>[2x]GSNRRLQQTQAQVDEVVDIMRVNVDKVLERDQKLSELDDRADALQAGASQFETSAAKLKRKYW;>[2x]ALSEIETRHSEIIKLENSIRELHDMFMDMAMLVESQGEMIDRIEYNVEHAVDYVERAVSDTKKAVK;>[2x]NELEEMQRRADQLADESLESTRRMLQLVEESKDAGIRTLVMLDEQGEQLDRVEEGMNHINQDMKEAEKNLKDLGK;>ARENEMDENLEQVSGIIGNLRHMALDMGNEIDTQNRQIDRIMEKADSNKTRIDEANQRATKMLG[2x];>[3x]KLGKLQYSLDYDFQNNQLLVGIIQAAELPALDMGGTSDPYVKVFLLPDKKKKFETKVHRKTLNPVFNEQFTFKVPYSELGGKTLVMAVYDFDRFSKHDIIGEFKVPMNTVDFGHVTEEWRDLQSAEKEEQEKLGDICFSLRYVPTAGKLTVVILEAKNLKKMDVGGLSDPYVKIHLMQNGKRLKKKKTTIKKNTLNPYYNESFSFEVPFEQIQKVQVVVTVLDYDKIGKNDAIGKVFVGYNSTGAELRHWSDMLANPRRPIAQWHTLQVEEEVDAMLAV

We subsequently successfully applied our methods to the previously unknown crystal structure of the complex between synaptotagmin-1 (Syt1) and the neuronal SNARE complex, which mediates the fusion of synaptic vesicles with the synaptic membrane and is essential for Ca2+-dependent neurotransmitter release. The Syt1–SNARE complex crystallizes in two distinct crystal forms with morphologies that were indistinguishable by inspection of the crystals.

We reprocessed the XFEL diffraction data of the Syt1–SNARE complex at 3.5 Å resolution to take advantage of all improvements implemented since the original publication. The XFEL data were collected at the X-ray Pump Probe (XPP) endstation of the Linac Coherent Light Source (LCLS) at the SLAC National Accelerator Laboratory, using a goniometer-based fixed target sample delivery station and an automatic sample loading system similar to the setup used for conventional synchrotron data collection at SSRL (Cohen et al., 2002, 2014). We then correlated each indexed image with the crystal it was obtained from, and identified 72 crystals that belonged to the 'long unit cell' (a = 69.4 Å, b = 170.8 Å, c = 291.2 Å, α = β = γ = 90°) crystal form. Of the 362 'long unit cell' diffraction images, 328 images were successfully integrated using the wide grid search parameters, while 34 images could not be integrated for a variety of reasons (insufficient number of Bragg reflections, poor diffraction quality, or un-resolvable multiple lattices). The remaining 313 integrated diffraction images were included in the final merged XFEL data set. Even though only 313 XFEL diffraction images were used in the final merged data set, it had high completeness (97.8%) and good multiplicity (6.1), along with reasonable merging statistics to 3.5 Å resolution. Re-refinement of the Syt1 – SNARE structure against the reprocessed XFEL data resulted in better atomic model Rwork / Rfree values (29.2% / 32.9% vs. 32.2% / 35.3%) than the originally published structure. Moreover, the reprocessed XFEL diffraction data produced slightly more interpretable electron density maps, which in a few cases allowed better modeling of side chain rotamers that were previously difficult to interpret. Additionally, more Ca2+ were visible in the XFEL-data derived maps (21 Ca2+) than in synchrotron-data derived maps (15 Ca2+).>GHMEQTHRAIFRFVPRHEDELELEVDDPLLAELQAEDYWYEAYNMRTGARGVFPAYYAIEVT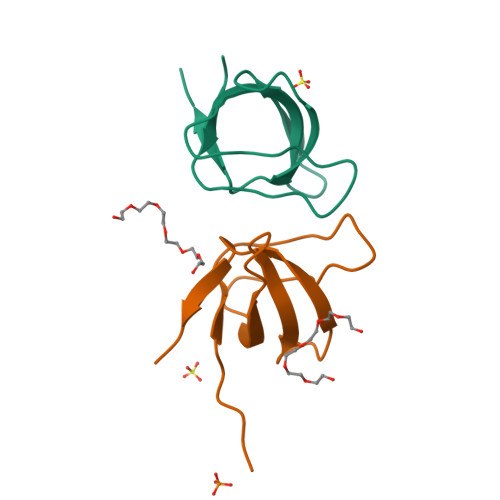K[4x]> SSIYARGRGGSSTDQPVANPYNTKEISLAAGLVQQTYCDSTENGLKIGDSELLYTMGEGYARQRVNIYHSPSLGIAVAIEGTNLFSLNSDLHDAKFWQEDPNERYIQYYPKGTKLMHGFQQAYNDLMDDIFTAVKKYKKEKNEKRVTVIGHSLGAAMGLLCAMDIELRMDGGLYKTYLFGLPRLGNPTFASFVDQKIGD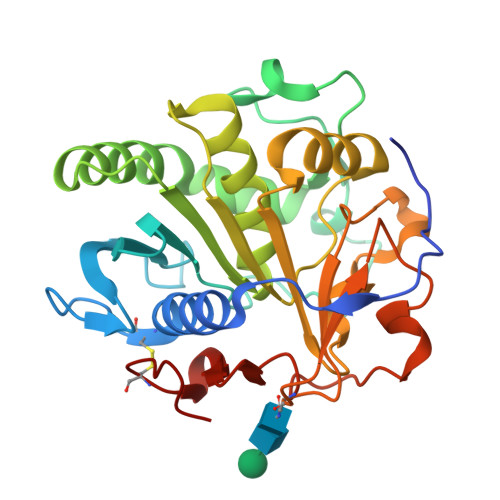KFHSIINGRDWVPTVPPRALGYQHPSDYVWIYPGNSTSAKLYPGQENVHGILTVAREFNDDDHQGIYFHTQIGAVMGECPAQVGAH>MTINYHELETSHGRIAVRESEGEGAPLLMIHGNSSSGAIFAPQLEGEIGKKWRVIAPDLPGHGKSTDAIDPDRSYSMEGYADAMTEVMQQLGIADAVVFGWSLGGHIGIEMIARYPEMRGLMITGTPPVAREEVGQGFKSGPDMALAGQEIFSERDVESYARSTCGEPFEASLLDIVARTDGRARRIMFEKFGSGTGGNQRDIVAEAQLPIAVVNGRDEPFVELDFVSKVKFGNLWEGKTHVIDNAGHAPFREAPAEFDAYLARFIRDCTQLEHHHHHH[2x]

N-Acyl homoserine lactonases (AHL-lactonases) have important functions in decreasing pathogenicity by degrading AHLs. Unlike most AHL-lactonases, AidH is proposed to be a member of the α/β-hydrolase fold family. AidH contains a substrate-binding tunnel between the core domain and the cap domain. Taken together, the present results reveal the catalytic mechanism of the metal-independent AHL-lactonase, which is a typical acid–base covalent catalysis.

The crystal structure of wild-type AidH complexed with the product C4-HS (AidH–C4-HS) was determined at 1.09 Å resolution. Following the lactone-bond breakage of N-butanoyl homoserine lactone (C4-HSL), the reaction product C4-HS features newly formed hydroxyl and carboxyl groups. The C4-­HS contains the O atom derived from the water molecule. The new carboxyl group forms hydrogen bonds to Ser102 and His248. In addition, the new hydroxyl group shows a rotation of approximately 98° around the axis of the C—C bond, resulting in a stretched conformation, and perfectly stabilizes this conformation by forming a hydrogen bond to Tyr160, which shifts by 1.3 Å compared with the substrate–enzyme complex. Tyr160 clutches the substrate and the product at the active site and positions them in the correct conformation via hydrogen bonds. In addition to the catalytic triad residues, Tyr160 is suggested to play a key role in catalysis. The entrance to the substrate-binding tunnel is in the open state upon substrate or product binding. Moreover, the size of the entrance varies with different substrate acyl-chain lengths.>[2x]MAHHHHHHSSGLEVLFQGPMEMILEEKDASDWIYRGEGGANLVLAYAGSSPLFVGKVIRIQKARRNDKAIKNSNGVVSVLTSDEQHLWRENNELISSPNKEVLEQRYVQNVIIPLLGPKHVDAGVRVSVSKEF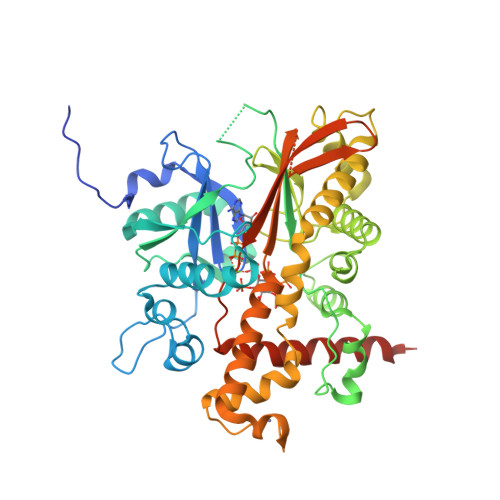LECVDKKVTKQRPLWRVNAANVDTSHDSALILNDHSLFSQGITSGGDCISVEIKPKCGFLPTSRFIGKENMLKTSVSRFKMHQLLKLEYIEISEESEYDPLDLFSGSKERVLEAIKALYSTPQNNFRVFLNGSLILGGSGESTGRTSPEIGYAFEDALKGFIQSEDGHRTECFLQLVSDAVYGSGVLDRLLEIQKLDKLDIEGAIHCYYDIINQPCPICKEGRPLEAELSLHALPLDESLKIVKEYLIAATAKDCSIMISFQSRNAWDSEPSGDYVSLKPTNQTFDYKVHFIDLSLKPLKRMESYYKLDKKIISFYNRKQKAENTAEQIGNSKPSHS>MVSAPSIDTPSATTFDFDSSVFKKEKVTLSGHDEYIVRGGRNLFPLLPDAFKGIKQIGVIGWGSQAPAQAQNLKDSLTEAKSDVVVKIGLRKGSNSFAEARAAGFSEENGTLGDMWETISGSDLVLLLISDSAQADNYEKVFSHMKPNSILGLSHGFLLGHLQSLGQDFPKNISVIAVCPKGMGPSVRRLYVQGKEVNGAGINSSFAVHQDVDGRATDVALGWSIALGSPFTFATTLEQEYKSDIFGERGILLGAVHGIVECLFRRYTESGMSEDLAYKNTVECITGVISKTISTKGMLALYNSLSEEGKKDFQAAYSASYYPSMDILYECYEDVASGSEIRSVVLAGRRFYEKEGLPAFPMGKIDQTRMWKVGEKVRSVRPAGDLGPLYPFTAGVYVALMMAQIEILRKKGHSYSEIINESVIEAVDSLNPFMHARGVSFMVDNCSTTARLGSRKW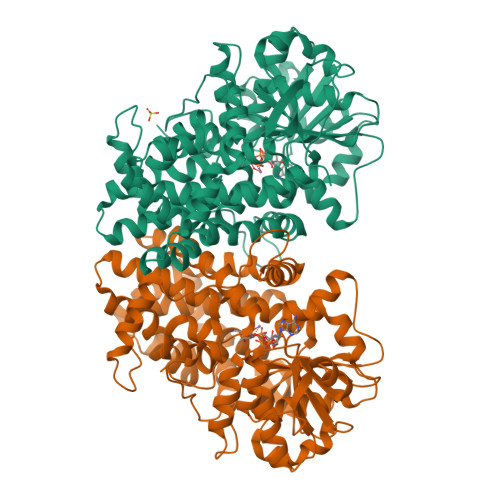APRFDYILSQQALVAVDNGAPINQDLISNFLSDPVHEAIGVCAQLRPSVDISVTADADFVRPELRQA[4x]> MRYLKIEKEKLVSCKKQEQEVQRIRRRKGNQKLNSIAKQQRVKRRDYQQNIKQNKEVKNPKKLIKQQIINKVKKRKKMFRGLTKFNKVFALNSFKNSLVAVPKANLNHVQNMLEENLKYDAQKYNDEVAVIQKTSRIYKPTYTIEFNREGEVLVYSA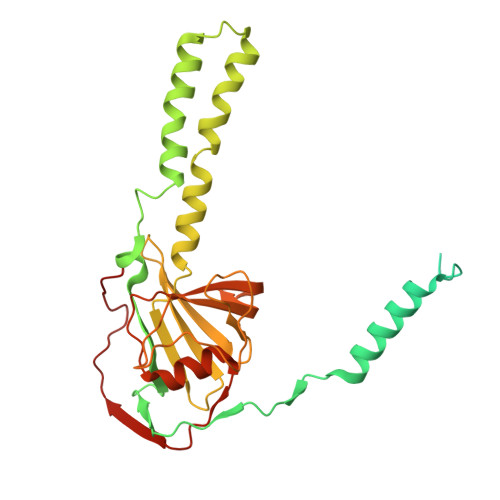DPIKNSVVYFKYPYVLYEAAIPLFIWAWIYNPLELSKNAVNSLLIYPNIAWIPRMWYWRSLQYKIQKMYLLRGGKVAKIETQSLAGDRFTSWVETYQFHPLTQDQKNFDNQDNAEFLEDEGQLKYELGVQLDNLQEMGTTSQDIVINFMKEGTVHHPELFEAIVKGYNIDTSDYVINTANNLRAREGNHNH> NCSKIHLSTKLLAVDFPAHFVKSISCQICEHILADPVETSCKHLFCRICILRCLKVMGSYCPSCRYPCFPTDLESPVKSFLNILNSLMVKCPAQDCNEEVSLEKYNHHVSSHKESKETLVHINKGGRPRQHLLSLTRRAQKHRLRELKIQVKEFADKEEGGDVKAVCLTLFLLALRARNEHRQADELEAIMQGRGSGLQPAVCLAIRVNTFLSCSQYHKMYRTVKAITGRQIFQPLHALRNAEKVLLPGYHPFEWQPPLKNVSSRTDVGIIDGLSGLASSVDEYPVDTIAKRFRYDSALVSALMDMEEDILEGMRSQDLDDYLNGPFTVVVKESCDGMGDVSEKHGSGPAVPEKAVRFSFTVMRITIEHGSQNVKVFEEPKPNSELCCKPLCLMLADESDHETLTAILSPLIAEREAMKSSELTLEMGGIPRTFKFIFRGTGYDEKLVREVEGLEASGSVYICTLCDTTRLEASQNLVFHSITRSHAENLQRYEVWRSNPYHESVEELRDRVKGVSAKPFIETVPSIDALHCDIGNAAEFYKIFQLEIGEVYKHPNASKEERKRWQATLDKHLRKRMNLKPIMRMNGNFARKLMTQETVDAVCELIPSEERHEALRELMDLYLKMKPVWRSSCPAKECPESLCQYSFNSQRFAELLSTKFKYRYEGKITNYFHKTLAHVPEIIERDGSIGAWASEGNESGNKLFRRFRKMNARQSKCYEMEDVLKHHWLYTS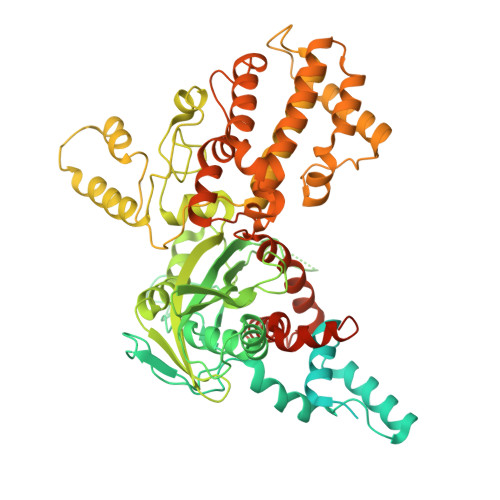KYLQKFMNAHNALKSSGFTMNSKETLGDPLGIEDSLESQDSME> YEVKFVEAYASLFKSRLSKLKRILRENPEISNVVDIGKLNYVSGDEEVTIIGLVNSKRETNRGLIFEVEDKTGIVKVFLPKDSEDYREAFKVLPDAVVAFKGFYSKKGIFFANKFYLPDVPLYRKQKPPLEEKVYAILISDIHVGSREFCEKAFLKFLEWLNGHVESKEEEEIVSRVKYLIIAGDVVDGIGIYPGQYSDLVIPDIFDQYEALANLLANVPEHITMFIGPGNADAARPAIPQPEFYKEYAKPIYKLKNAIIISNPAVIRLHGRDFLIAHGRGIEDVVSFVPGLTHHKPGLPMVELLKMRHLAPTFGGKVPIAPDPEDLLVIEEVPDLVQMGHVHVYDAVVYRGVQLVNSATWQAQTEFQKMVNIVPTPAKVPVVDVESARVVKVLDFSGWC;> MELPKEMEEYFEMLQREIDKAYEIAKKARAQGKDPSLDVEIPQATDMAGRVESLVGPPGVAKRIRELVKEYGKEIAALKIVDEIIEGKFGDLGSREKYAEQAVRTALAILTEGIVSAPIEGIANVKIKRNTWADNSEYLALYYAGPIRSSGGTAQALSVLVGDYVRRKLGLDRFKPSEKHIERMVEEVDLYHRAVTRLQYHPSPEEVRLAMRNIPIEITGEATDDVEVSHRDVPGVETNQLRGGAILVLAEGVLQKAKKLVKYIDKMGIEGWEWLKEFVEAKEKGEPKEEGKEESLAESTLEETKVEVDMGFYYSLYQKFKEEIAPSDKYAKEVIGGRPLFSDPSKPGGFRLRYGRSRASGFATWGINPATMILVDEFLAIGTQLKTERPGKGAVVTPVTTIEGPIVKLKDGSVLRVDDYNLALKVREDVEEILYLGDAVIAFGDFVENNQTLLPANYCEEWWILEFVKALKEIYEVHLEPFTENEEESIEEASDYLEIDPEFLKEMLRDPLRVKPPVELAIHFSEVLGIPLHPYYTLYWNSVEPKDVEKLWRLLKNYAEIEWSNFRGIKFAKKIVISQEKLGDSKRTLELLGLPHTVRDGNVIVDYPWAAALLTPLGNLNWEFMAKPLYATIDIINENNEIKLRDRGISWIGARMGRPEKAKERKMKPPVQVLFPIGLAGGSSRDIKKAAEEGKVAEVEIAFFKCPKCGHVGPEHLCPNCGTRKELLWVCPRCNAEYPESQAEGYNYTCPKCNVKLRPYAKRKIRPSELLNRAMENVKVYGVDKLKGVMGMTSGWKMPEPLEKGLLRAKNDVYVFKDGTIRFDATDAPITHFRPREIGVSVEKLRELGYTHDFEGKPLVSEDQIVELKPQDIILSKEAGRYLLKVAKFVDDLLEKFYGLPRFYNAEKMEDLIGHLVIGLAPHTSAGIVGRIIGFVDALVGYAHPYFHAAKRRNCDGDEDAVMLLLDALLNFSRYYLPEKRGGKMDAPLVITTRLDPREVDSEVHNMDIVRYYPLEFYEATYELKSPKELVGVIERVEDRLGKPEMYYGLKFTHDTDDIALGPKMSLYKQLGDMEEKVRRQLEVAKRIRAVDEHGVAEKILNSHLIPDLRGNLRSFTRQEFRCVKCNTKFRRPPLNGKCPVCGGKIVLTVSKGAIEKYLGTAKMLVTEYNVKNYTRQRICLTERDIDSLFENVFPETQLTLIVNPNDICQRLVMARTGEVNKSGLLENLSNGSKKTEKAEKAEKPRKKSDEKPKKKRVISLEEFFSRKSK

PolD is an unusual archaeal replicative DNA polymerase (DNAP) in that it has all the functional properties of a replicative DNAP but with a catalytic core reminiscent of an RNA polymerase (RNAP). PolD is a heterodimeric replicative DNAP composed of a large catalytic subunit (DP2) and a smaller subunit with 3′-5′ proofreading exonuclease activity (DP1). A characteristic of PolD is that the exonuclease and polymerase active sites are hosted by two distinct subunits. Indeed, PolD has been shown to share an unexpected structural homology with the “two-double-psi β-barrel” (DPBB) family of RNAPs, which includes multisubunit transcriptases from all domains of life, homodimeric RNA silencing pathway RNAPs, and atypical RNAPs encoded by some viruses.

We now describe the cryo–electron microscopy (cryo-EM) structure of a DNA-bound heterodimeric DP1–DP2 PolD complex from the archaeon Pyrococcus abyssi, revealing a unique DNA-binding site. The PolD exonuclease-deficient variant (DP1 H451A) was incubated with a 15-mer primed DNA duplex with a 5-nt overhang, mimicking DNA replication intermediates, to prepare samples for cryo-EM. The best electron density was obtained from a subset of 8,774 particles isolated from iterative 3D classifications and yielding to a density map at an overall resolution of 7.1 Å. In the DNA-bound PolD structure, a 15-mer/16-mer primer/template duplex B-form DNA was docked in the cryo-EM density, guided by the unambiguous density for the duplex region, showing minor and major grooves. PolD shows a claw-shaped active site, at the center of which is the two-DPBB catalytic core and at the edge of which are three zinc-binding modules named the Zn-I, Zn-II, and Zn-III domains. The DNA substrate is cradled between a bipartite clamp domain, named 1 and 2, emanating from DPBB-1 and DPBB-2, respectively. The clamp domain is barricaded from one side by a globular domain (85–283) located in the N-terminal region of DP2, which is ideally located to orient the DNA template in the active site. PolD has evolved a specific bipartite clamp domain, which completely surrounds the DNA duplex. In total, the Zn-III domain of clamp-1; loop-I, loop-II, and loop-III of clamp-2; and several residues of the two-DPBB catalytic center contribute conserved basic residues that form a circular clamp that binds about one turn of helix (10–12 base pairs) of the nascent DNA duplex. Comparison of the cryo-EM PolD structure with the DP2 (1–1061) crystal structure reveals that the association with DP1 is required for rearranging the DP2 catalytic core into an active conformation.> DEHEHCCSEEDHRIVQKQWDILWRDTESSKIKIGFGRLLLTKLAKDIPEVNDLFKRVDIEHAEGPKFSAHAL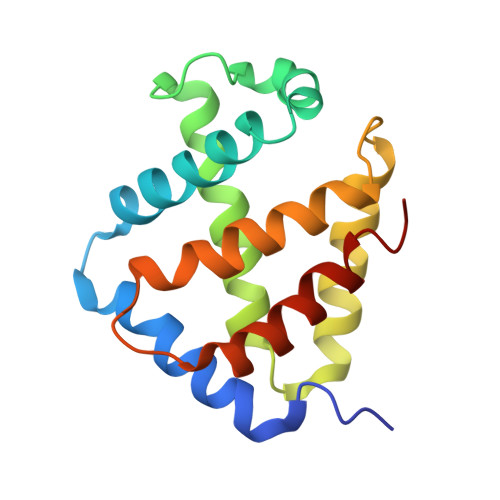RILNGLDLAINLLDDPPALDAALDHLAHQHEVREGVQKAHFKKFGEILATGLPQVLDDYDALAWKSCLKGILTKISSRLNA>[6x]MSLDTGVTSVMFVERSLNEIRFWSRIMKEHSFFLRLGFRCEDTQLIEEANQFYRLFEHIEQIAHSYTNETDPEQIKRFNAEVQQAATNIWGFKRKILGLILTCKLPGQNNFPLLVDHTSREADYFRKRLIQLNEGKLDALPDAII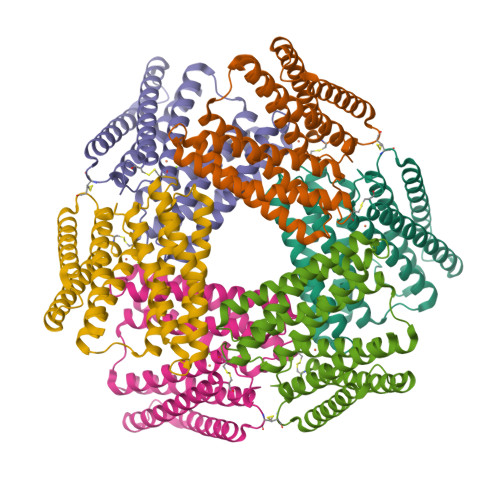KENVFFLRIMADHAKFIGHLLDPSERKLVDTARNFSNDFDELMYQAIDLESMKPQSQTAPLLDQFLDQNRVSVASLRDFKKTARDLIEQCKIKSIIHPLLADHVFREADRFLEIIDMYDVHLTNIQSQPREGHHHHHH> MAMRQCAIYGKGGIGKSTTTQNLVAALAEMGKKVMIVGCDPKADSTRLILHSKAQNTIMEMAAEAGTVEDLELEDVLKAGYGGVKCVES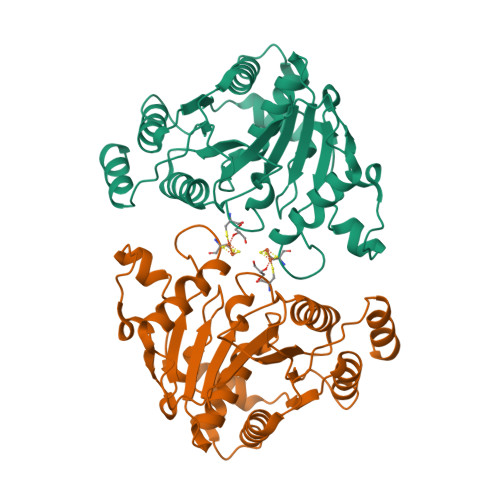GGPEPGVGCAGRGVITAINFLEEEGAYEDDLDFVFYDVGDVVCGGFAMPIRENKAQEIYIVCSGEMMAMYAANNISKGIVKYANSGSVRLGGLICNSRNTDREDELIIALANKLGTQMIHFVPRDNVVQRAEIRRMTVIEYDPKAKQADEYRALARKVVDNKLLVIPNPITMDELEELLMEFG>MGNCLDSSAKVDNSNHSPHANSASSGSKVSSKTSRSTGPSGLSTTSYSTDSSFGPLPTLRTEGEILSSPNLKAFTFNELKNATKNFRQDNLLGEGGFGCVFKGWIDQTSLTASRPGSGIVVAVKQLKPEGFQGHKEWLTEVNYLGQLSHPNLVLLVGYCAEGENRLLVYEFMPKGSLENHLFRRGAQPLTWAIRMKVAVGAAKGLTFLHEAKSQVIYRDFKAANILLDADFNAKLSDFGLAKAGPTGDNTHVSTKVIGTHGYAAPEYVATGRLTAKSDVYSFGVVLLELISGRRAMDNSNGGNEYSLVDWATPYLGDKRKLFRIMDTKLGGQYPQKGAFTAANLALQCLNPDAKLRPKMSEVLVTLEQLESVAKPGTKHTQMESPRFHHSSVMQKSPVRYSHDRPLLHMTPGASPLPSYTQSPRVR[5x];>[5x]MKKQYLKSGSGTRKEKDKAKRWFLDNGSIFLRELVADCNGKSIPIRSFSPEQILKATNNFDSSCFVSQDVYYKWYRGEIEDRSYMIKRFSEDEITGKRHRVKEVYNDIVLSARMSNHSNFLQLLGCCLEFPFPVLVFEFAEHGAMNQRGGVIVNGEESLLPWSVRLKIGKEIANAVTYLHTAFPKIIIHRDVKPMHVFLDKNWTAKLSDLSFSISLPEGKSRIEAEWVLGTFGYIDPLYHKTCFVTEYTDVYSFGICLLVIITGKPAIMTISDGDLQGILSLVRELCENGKLDEVIDPRLMKDITSGQRLQVEACVVLALRCCKERDEDRPKMIQVAKELKQIEASLKNSS;>[5x]MVDAVVTVFLEKTLNILEEKGRTVSDYRKQLEDLQSELKYMQSFLKDAERQKRTNETLRTLVADLRELVYEAEDILVDCQLADGDDGNEQRSSNAWLSRLHPARVPLQYKKSKRLQEINERITKIKSQVEPYFEFITPSNVGRDNGTDRWSSPVYDHTQVVGLEGDKRKIKEWLFRSNDSQLLIMAFVGMGGLGKTTIAQEVFNDKEIEHRFERRIWVSVSQTFTEEQIMRSILRNLGDASVGDDIGTLLRKIQQYLLGKRYLIVMDDVWDKNLSWWDKIYQGLPRGQGGSVIVTTRSESVAKRVQARDDKTHRPELLSPDNSWLLFCNVAFAANDGTCERPELEDVGKEIVTKCKGLPLTIKAVGGLLLCKDHVYH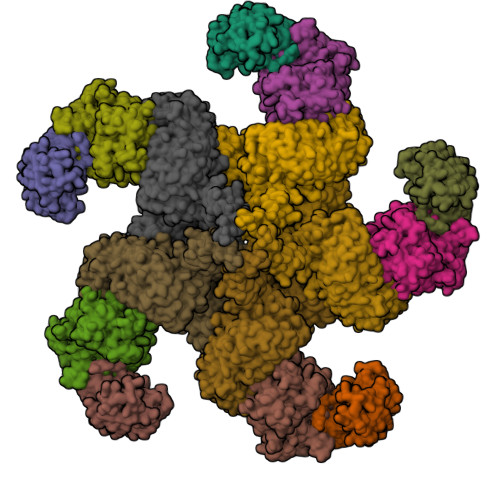EWRRIAEHFQDELRGNTSETDNVMSSLQLSYDELPSHLKSCILTLSLYPEDCVIPKQQLVHGWIGEGFVMWRNGRSATESGEDCFSGLTNRCLIEVVDKTYSGTIITCKIHDMVRDLVIDIAKKDSFSNPEGLNCRHLGISGNFDEKQIKVNHKLRGVVSTTKTGEVNKLNSDLAKKFTDCKYLRVLDISKSIFDAPLSEILDEIASLQHLACLSLSNTHPLIQFPRSMEDLHNLQILDASYCQNLKQLQPCIVLFKKLLVLDMTNCGSLECFPKGIGSLVKLEVLLGFKPARSNNGCKLSEVKNLTNLRKLGLSLTRGDQIEEEELDSLINLSKLMSISINCYDSYGDDLITKIDALTPPHQLHELSLQFYPGKSSPSWLSPHKLPMLRYMSICSGNLVKMQEPFWGNENTHWRIEGLMLSSLSDLDMDWEVLQQSMPYLRTVTANWCPELESFAIEDVGFRGGVWMKTPLHRT> MPSEQRGQHRSGYGLGLSTRTQVTGYQFLARRTAMALTRWRVRMEVEPGRRQVLAVVASVSAAGVICLGALLWSFISPSGQMGESPIIADRDSGALYVRVGDTLYPALNLASARLIAGRAENPHKVRSSQIAEQPHGPMVGIPGAPSDISPTSPASSSWLVCDAVTAAQGVGAPASVTVTVIDGTPDLSGRRHVLSGSDAVVLRYGNDTWVIRQGRRSRIDAANRAVLLPLGLTPEQVKQASPMSRALYDALPVGPELAVPKVPDAGKPANFPGAPAPVGAVLVTPQISGPQQYSVVLPDGVQTISPIVAQILQNAGTPAGSMPVVVAPATLARMPVVHGLDLSAYPDSPLNVVNMKENPATCWWWEKTAGEERARTQVVSGPTVPIATSDTNKVVSLVKADNTGREADRVYYGPNYANFVVVTGNDPAASTAESLWLLSKSGVRFGVDNSREARTALGLTSTPSPAPWVALRLLAPGPMLSRADALVRHDTLPTDTNPAELAVPK;> MKQGFARPTPERAPVVKPENIVLPTPLSVPPPEGKPWWLVVVGVLVVGLLVGMVGMTVASGSRLFLGAGAIFPIFMIGGVAMMMFGGRFGGQQQMSRPKLDAMRAQFMLMLDMLRETAQESADSMDANYRWFHPAPTTLAAAVGSSRMWERQPDGKDLNFGVVRVGVGMTRPEVTWGEPQNMPTDIELEPVTGKALQEFGRYQSVVYNLPKMVSLLVEPWYSLVGEREQVLGLTRAIICQLAFSHGPDHVQMIVVTSDPDRWDWVKWIPHFGDPRRRDAAGNARMVYTSVREFATEQAELFAGRGSFTPRHASSSAETPTPHHVIISDIEDPQWEYVISSEGVDGVTFFDLTGSPLWTGAPQRVLRFTDSAGVIETLPRDRDTWMVIDDNAWFFALADQMSEADAEQFAHQMAHWRLAEAYEEIGQRVVQLGARDILSYYGIDDAGEIDFNTLWSGSGRRDLLSRSRLRIPFGNRADNGELLFLDMKSLDEGGDGPHGVMSGTTGSGKSSLVRTVIASLMLAHPPEELQFVLADLKGGSAVKPFDGVPHVSRIITDLEDDQALMERFLEAMWGEIARRKEICFSAGVDGAKEYNELRARMKARGEDMPPLPMLVVVIDEFYEWFRIMPTAVDVLDSIGRQGRAYWVHLMMASQTIESRAEKLMENMGYRLVLKAQTAGAAQAAGVPNAVNLPSQAGLGYFRKSGDEIIRFQAEYLWRDYRRGSSYDGEEQAPLTHSVDYIRPQLFTTAFAPLEVSVSGPDGQSALPQVVDGEAVNGHRGGDDVDEEEEALRTPKVGTVIIDQLRQIDFEPYRLWHPPLDVPVPIDELVNRFLGRPWQQDYGTAKNLVFPIGIIDRPYKHDQPPWTVDTSGAGANVLILGAGGAGKTTALQTLICAAALTHTPEQVQFYCLAYSGTALTTVANLPHVGGVSGPTDPYGVRRTVAEVLGLVRDRKRSFLEYDVPSMEVFRRRKFGGEPGGVPDDGFGDVYLVIDNYRALAEENEVLIEQVNQIINQGPSFGVHVVATADRESELRPPVRSGFGSRVELRLAAVEDAKLVRSRFAKDVPPKPGRGMVAVNYVRLDSDPQAGLHTLVARPALGSTPDAVFESDSVAAAVRQVAAGEARPVRRLPARFGLDQLRQVAAADRRQGVGAGGIAWAISELDLQPVYLNFADNAHLMVTGRRECGRTTTLATIMSEIGRIYAPGASTAPPTSRPSAQVWLVDPRRQLLTVLGSDYVEKFAYNLDGVAAMMDDLAAALARREPPPGLSAEELLSRSWWSGPEIFLIIDDIQQLPPGFDSPLHKAAPWVTRAADVGLHVFVTRTFGGWSSAGSDPILRALHQANAPLLVMDADPDEGFIRGKMKGGPLPRGRGLLMAEDTGVFVQVAATDLRR;>MTAIVEAPQPGAEAIASPQAAVVAIMAADVQIAVVLDAHAPISVMIDPLLKVVNTRLRELGVAPLEAKGRGRWMLCLVDGTPLRPNLSLTEQEVYDGDRLWLKFLEDTEHRSEVIEHISTAVATNLSKRFAPIDPVVAVQVGATMVAVGVLLGSALLGWWRWQHESWLPAPFAAVIAVLVLTVATMILARSKTVPDRRVGDILLLSGLVPLAVAIAATAPGPVGAPHAVLGFGVFGVAAMLVMRFTGRRLGVYTALVTLCAAATAAGLARMVLLTSAVTLLTCVLLACVLMYHGAPALSRWLSGIRLPVFPSATSRWVFEARPDLPTTVVVSGGGQPTLEGPASVRDVLLRAERARSFLTGLLVGLGVLTVVCLAGLCDPHAGRRWLPLLLAAFTFGFLILRGRSYVDRWQAITLAATAVLIIAAVAVRYVLVSGSPAVLSAGVAVLVLLPAAGLTAAAVVPNTIYSPLFRKIVEWIEYLCLMPIFPLALWLMNVYEAIRYR[2x];> MRAQRRFGLDLSWPRLTGVFLIDVAVLALVSHLPDAWQANHIAWWTGVGVAVLVTIVAVVTYRRTPLACALVARVLDRFVDPEMTLTEGCTPALDHQRRFGHDVVGIREYQGQLVAVVTVEGHEEAPSGRHRNRDAAPAWLPVEAVAARLRQFDVRLDAIDIVSVGTRRTSGRDDVSDVGVDDTGPVDARQPLDEHHTWLVLRMDPQRNVAAVAARDSVAATLAAATERLAHDLNGRRWTARPLTSSEIDDMDATVLAGLQPAHVRPRRRRLKYKQPEGYKEFVTSFWVSPRDITSETLERLWLPDTEATAVTVRLRPRHGGVEVSAWVRYHSSRRLRRSVWGGLNRLTGRQLDAVCASMPVPTRRPRLVVPARELHDGEELAVLVGQAPAPSPSPAAAR

The ESX-5 type VII secretion system is a membrane-spanning protein complex key to the virulence of mycobacterial pathogens. Key to their pathogenicity is the secretion of a wide range of virulence proteins via type VII secretion systems (T7SSs). The ESX-5 T7SS is found almost exclusively in slow growing, pathogenic mycobacteria and plays a key role in nutrient uptake and immune modulation during an infection. The importance of ESX-5 and other ESX secretion systems (ESX-1 to ESX-4) for the virulence of mycobacterial pathogens makes these membrane-spanning machineries a key target for the development of novel therapeutics.

We therefore generated two new maps imposing C6 symmetry for modeling these regions: a global map with a 3.4-Å resolution and a locally refined map of the cytosolic part of the protomeric units at 3.0-Å resolution. Because of the observed sixfold symmetry of the TM and cytosolic segments of the ESX-5 complex, we first defined its overall arrangement as consisting of six identical protomeric subcomplexes. Within each protomeric unit, EccD5 was observed to assume an elliptical ring-shaped dimer composed of 22 (11 per EccD5 monomer) TM helices (TMHs) forming the core of the protomer. We observed that one of the EccD5 molecules is proximal and the second one is distal to the central pore, and we annotated them as EccD5-1 and EccD5-2, respectively. We noted that the EccD5 ring-like arrangement is further supported by interactions at the cytoplasmic face formed by TMH6 and the elongated TMH7, connected by an extended loop. Because of the approximate twofold symmetry of each EccD5 dimer, TMH11 of EccD5-2 was found most distal, and TMH11 of EccD5-1 is the closest to the central pore. Both TMH11 helices displayed a distinct diagonal orientation with respect to the remaining EccD TMHs and the pore axis (see below). In our model, contacts between TMH11 from EccD5-1 and the only EccB5 TMH establish a scaffold for the central pore. Besides these interactions at the interface between the membrane and the cytoplasm (membrane cytoplasm inset), we observed several specific electrostatic interactions of the EccC5 stalk domain with the N-terminal EccB5 helix, situated parallel to the membrane. In our structure, the DUF domain was the most distal rigid component at the cytosolic face of the ESX-5 complex.>[2x]MKKRLLLPLFAALCLSQIAHADEGMWLMQQLGRKYAQMKERGLKMKEYDLYNPNGTSLKDAVVLFDGGCTGEVVSDRGLVLTNHHCGYDMIQAHSTLEHNYLENGFWAMREADELPNKDISVVFIDKIEDVTDYVKKELKAIKDPNSMDYLSPKYLQKLADKKAGKNFSAKNPGLSVEIKAFYGGNLYLMFTKKTYTDVRLVGAPPSSIGKFGADTDNWIWPRHTGDFSIFRIYADKNGNPAPYSEDNVPLKPKRFFNISLGGVQENDYAMIMGFPGTTHRYFTASEVDEWKSIDNDIRIRMRDIRQGVMLREMLADPQIKIMYSAKYAASQNAYKRAIGANWAIKTRGLRQNKQAMQDRLIAWGAKQGTPRYEEAVHEIDATVAKRADLRRRYWMIEEGIIRGIEFARS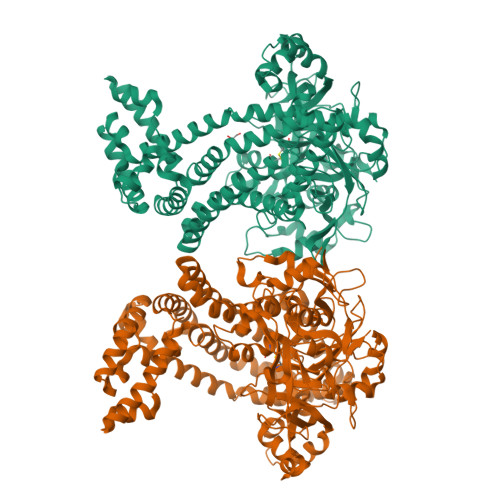PIPTEDETKALQGNDASARKEAIDKIRTRYSKFANKDYSAEVDKKVAVAMLTEYLKEIPYENLPLHLRLVKDRFAGDVQAYVDDIFARSVFGSEAQFDAFAAVPSVEKLAEDPMVLFASSVFDEYRKLYNELRPYDDPILRAQRTYIAGLLEMDGDQDQFPDANLTLRFTYGQVKGYSPRDNVYYGHQTTLDGVMEKEDPDNWEFVVDPKLKAVYERKDFGRYADRSGRMPVAFCATTHTTGGNSGSPVMNANGELIGLNFDRNWEGVGGDIQYLADYQRSIIVDIRYVLLVIDKVGGCQRLLDEMNIVP> GASSLKDEVPTETSEDFGFKFLGQKQILPSFNEKLPFASLQNLDISNSKSLFVAASGSKAVVGELQLLRDHITSDSTPLTFKWEKEIPDVIFVCFHGDQVLVSTRNALYSLDLEELSEFRTVTSFEKPVFQLKNVNNTLVILNSVNDLSALDLRTKSTKQLAQNVTSFDVTNSQLAVLLKDRSFQSFAWRNGEMEKQFEFSLPSELEELPVEEYSPLSVTILSPQDFLAVFGNVISETDDEVSYDQKMYIIKHIDGSASFQETFDITPPFGQIVRFPYMYKVTLSGLIEPDANVNVLASSCSSEVSIWDSKQVIEPSQDSERAVLPISEETDKDTNPIGVAVDVVTSGTILEPCSGVDTIERL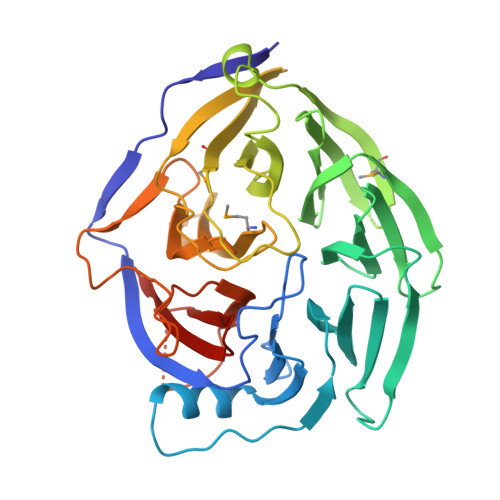PLVYILNNEGSLQIVGLFHVAAIKS GLUTATHIONYLSPERMIDINE | C17 H34 N6 O5 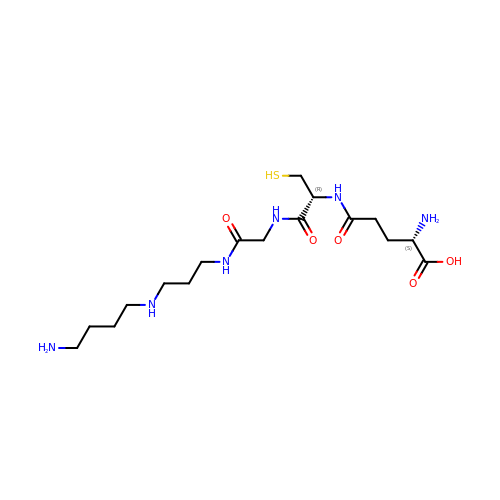S | NEDQLXHBVHSKNV-STQMWFEESA-N> HEVPSGP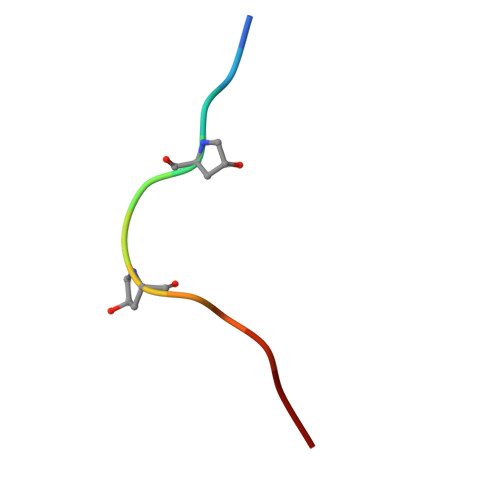NPISN> GAMPPRRTIRFSVDRPF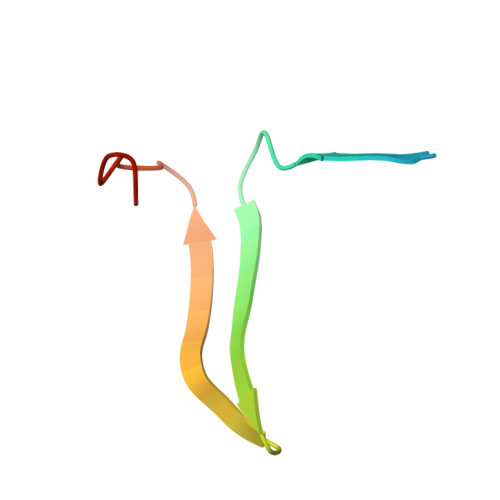HIVVRRRGAILFLGSIADPHDPGPAQ>[3x]SNAERRLCAILAADMAGYSRLMERNETDVLNRQKLYRRELIDPAIAQAGGQIVKTTGDGMLARFDTAQAALRCALEIQQAMQQREEDTPRKERIQYR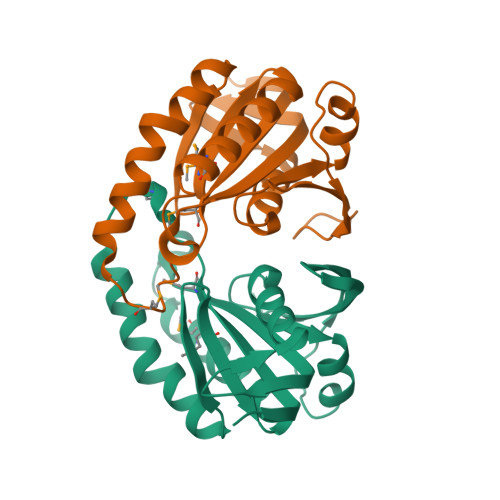IGINIGDIVLEDGDIFGDAVNVAARLEAISEPGAICVSDIVHQITQDRVSEPFTDLGLQKVKNITRPIRVWQWVPDADRDQSHDPQPSHVQH> MKKHHHHHHDNATDDPVDLVYAAEKIIQKRVKKGVVEYRVKWKGWNQRYNTWEPEVNILDRRLIDIYEQ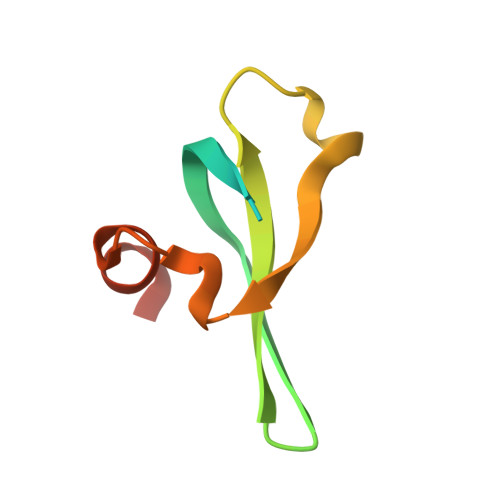TNK>[2x]MSVIEVTDENFEQEVLKSDK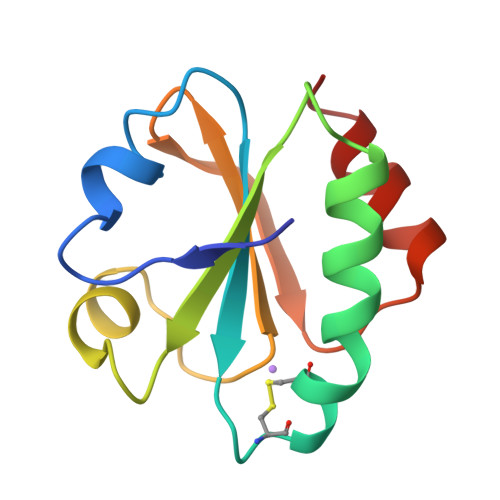PVLVDFWAPWCGPCRMIAPIIEELAKEYEGKVKVVKVNVDENPNTAAQYGIRSIPTLLLFKNGQVVDRLVGAQPKEALKERIDKHL4-(2-amino-5,6,7,8-tetrahydropyrimido[4',5':3,4]cyclohepta[1,2-b]indol-11-yl)-2-methylbut-3-yn-2-ol | C20 H20 N4 O | 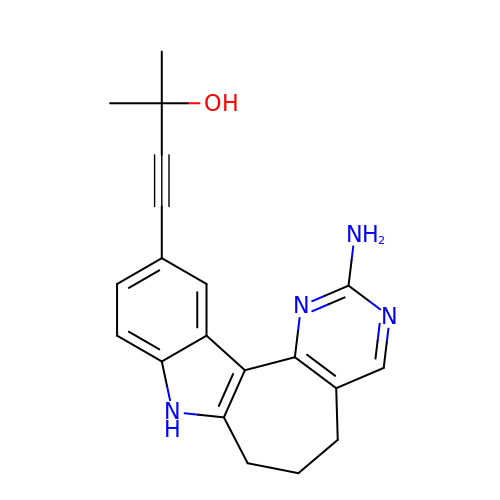DGLFSNZWRYADFC-UHFFFAOYSA-N> CVTQLLKDTCFEGGDITTVFTPSAKYCQVVCTYHPRCLLFTFTAESPSEDPTRWFTCVLKDSVTETLPRVNRTAAISGYSFKQCSHQISACNKDIYVDLDMKGINYNSSVAKSAQECQERCTDDVHCHFFTYATRQFPSLEHRNICLLKHTQTGTPTRITKLDKVVSGFSLKSCALSNLACIRDIFPNTVFADSNIDSVMAPDAFVCGRICTHHPGCLFFTFFSQEWPKESQRNLCLLKTSESGLPSTRIKKSKALSGFSLQSCRHSIPVFCHSSFYHDTDFLGEELDI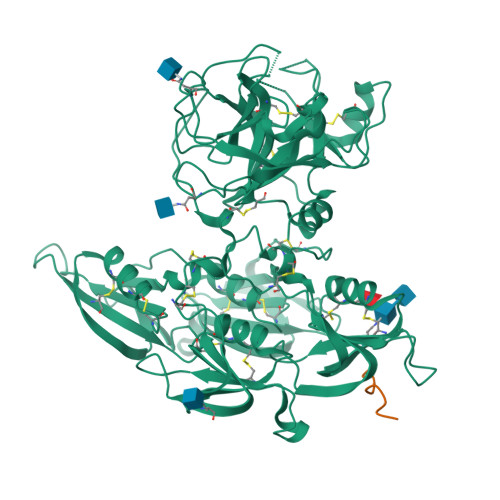VAAKSHEACQKLCTNAVRCQFFTYTPAQASCNEGKGKCYLKLSSNGSPTKILHGRGGISGYTLRLCKMDNECTTKIKPRIVGGTASVRGEWPWQVTLHTTSPTQRHLCGGSIIGNQWILTAAHCFYGVESPKILRVYSGILNQSEIKEDTSFFGVQEIIIHDQYKMAESGYDIALLKLETTVNYTDSQRPICLPSKGDRNVIYTDCWVTGWGYRKLRDKIQNTLQKAKIPLVTNEECQKRYRGHKITHKMICAGYREGGKDACKGDSGGPLSCKHNEVWHLVGITSWGEGCAQRERPGVYTNVVEYVDWILEKTQAV;> HIYPDFPTD> NATTPTMQSTSLLTEHLGYPPISLVDDIINAVNEIMYKCTNAMEKYLMQRNIIGKKDFSDEIKIGTAKLESLLENSVDKNFDKLELYVLRNILS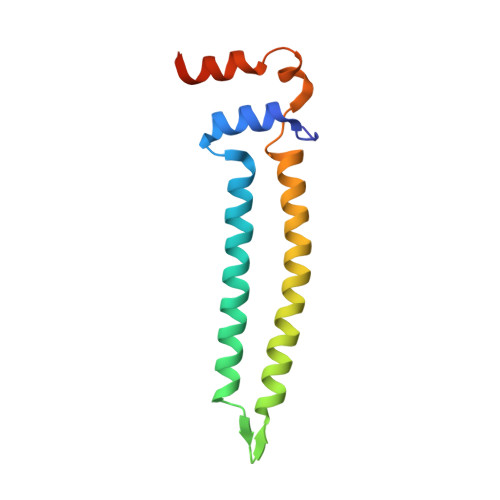IPSDLLEENRFRLLHHEKLVLTDSATR> GGGLGLIKSL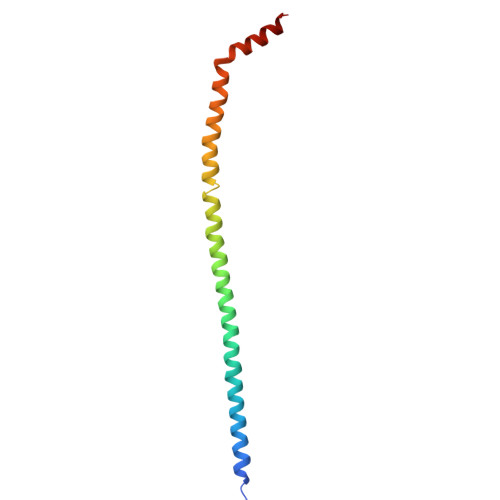AEKEKQLLERLEAAKKEAEERVKRAEAEAKALLEEAEAKAKALEAQYRERERAETEALLARYRERAEAEAKAVREKAMARLDEAVALVLKEVLP> MHHHHHHSSGLEVLFQGPGSVPLPAGWEMAKTSSGQRYFLNHNDQTTTWQDPRKAMLSQLNVPAPASPAVPQTLMNSASGPLPDGW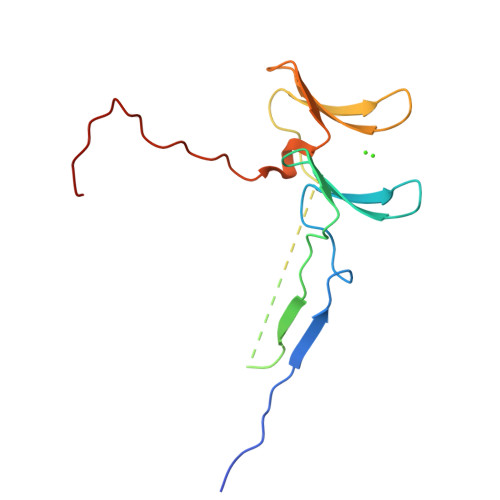EQAMTQDGEVYYINHKNKTTSWLDPRDRPPPYVAPPSYEGPHRTLG>GSHMD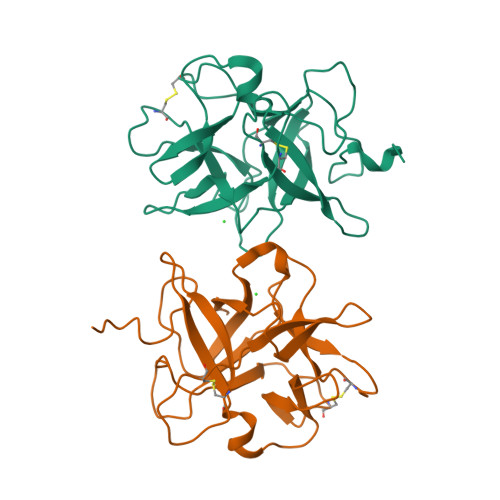DDLVDAEGNLVENGGTYYLLPHIWAHGGGIETAKTGNEPCPLTVVRSPNEVSKGEPIRISSPYRIRFIPRGSLVALGFANPPSCAASPWWTVVDSPQGPAVKLSQQKLPEKDILVFKFEKVSHSNIHVYKLLYCQHDEEDVKCDQYIGIHRDRNGNRRLVVTEENPLELVLLKAKSETASSH[2x]> GPLGSMRRSKADVERYIASVQGSTPSPRQKSMKGFYFAKLYMEAKEYDLAKKYICTYINVQERDPKAHRFLGLLYELEENT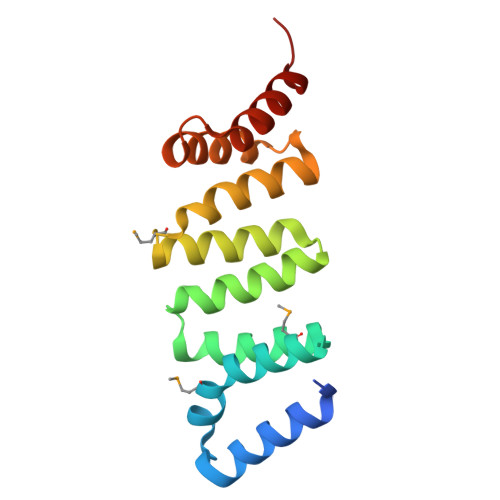DKAVECYRRSVELNPMQKDLVLKIAELLCKNDVTDGRAKYWVERAAKLFPGSPAVYKLKEQLLDCEGED> MTVFFKTLRNHWKKTTAGLCLLTWGGHWLYGKHCDNLLRRAACQEAQVFGNQLIPPNAQVKKATVFLNPAACKGKARTLFE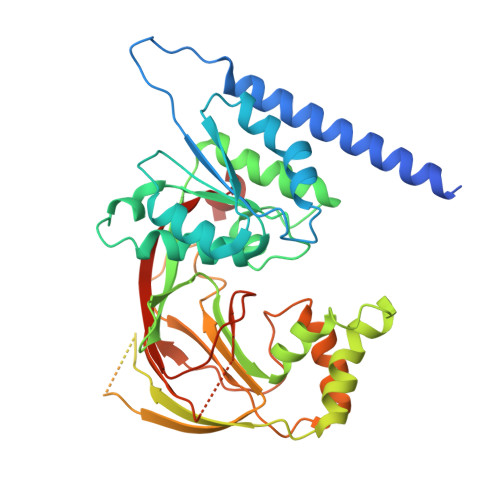KNAAPILHLSGMDVTIVKTDYEGQAKKLLELMENTDVIIVAGGDGTLQEVVTGVLRRTDEATFSKIPIGFIPLGETSSLSHTLFAESGNKVQHITDATLAIVKGETVPLDVLQIKGEKEQPVFAMTGLRWGSFRDAGVKVSKYWYLGPLKIKAAHFFSTLKEWPQTHQASISYTGPTERPPNEPEETPVQRPSLYRRILRRLASYWAQPQDALSQEVSPEVWKDVQLSTIELSITTRNNQLDPTSKEDFLNICIEPDTISKGDFITIGSRKVRNPKLHVEGTECLQASQCTLLIPEGAGGSFSIDSEEYEAMPVEVKLLPRKLQFFCDPRKREQMLTSPTQ> NSINFDNPVYQKT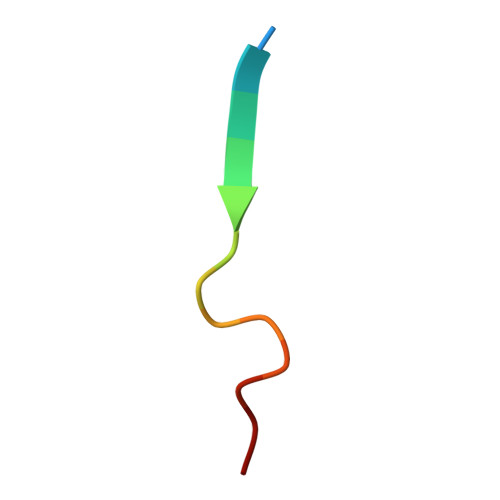T>STHFDVIVVGAGSMGMAAGYQLAKQGVKTLLVDAFDPPHTNGSHHGDTRIIRHAYGEGREYVPLALRSQELWYELEKETHHKIFTKTGVLVFGPKGESAFVAETMEAAKEHSLTVDLLEGDEINKRWPGITVPENYNAIFEPNSGVLFSENCIRAYRELAEARGAKVLTHTRVEDFDISPDSVKIETANGSYTADKLIVSMGAWNSKLLSKLNLDIPLQPYRQVVGFFESDESKYSNDIDFPGFMVEVPNGIYYGFPSFGGCGLKLGYNTFGQKIDPDTINREFGVYPEDESNLRAFLEEYMPGANGELKRGAVCMYTKTLDEHFIIDLHPEHSNVVIAAGFSGHGFKFSSGVGEVL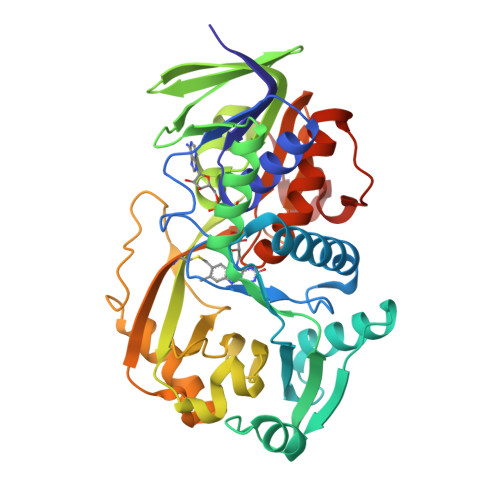SQLALTGKTEHDISIFSINRPALKESLQKTTI[2x]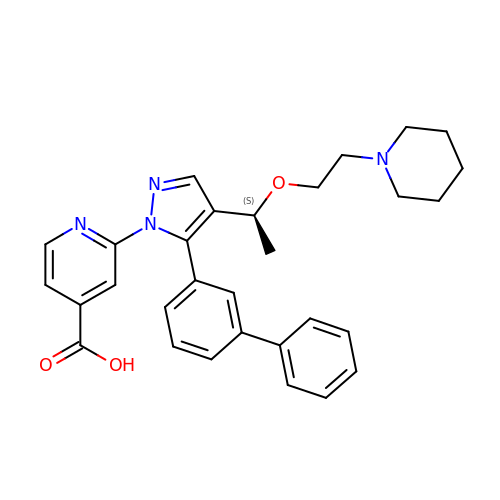2-[5-([1,1'-biphenyl]-3-yl)-4-{(1S)-1-[2-(piperidin-1-yl)ethoxy]ethyl}-1H-pyrazol-1-yl]pyridine-4-carboxylic acid | C30 H32 N4 O3 | LYCMOOQJGJJWEY-QFIPXVFZSA-N> MFLNRLVKETSKAKRLFSMAQNNFARAGPYNPNRYKDYYIPRTLPKNEEIVEFVQSQHSVPASPIRNQRHINPVRESGPLPSYDGTYTMEDIRAVFYNTTVGRDYCYCQMDPEEIMRRVPGITRKEAEFITKLGLSPQEQVDFAYIAYNIGLDIFYF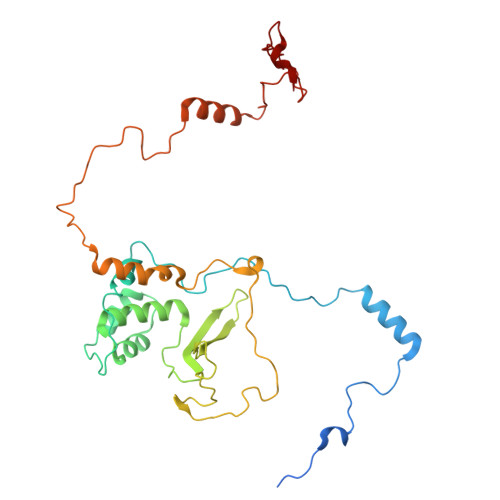TNQMFVARQVVTNSKGEKVEVLWNAQCYEDIAQLNVGFAPVLESVDYHWEIFLWADPPIKPNNDFDLNVPCTWFEYEQEWWMESCIQEDQFNLPEDERPYNTPRNPHCRKELWRSQDALQEEELMVNENWYPKNTQYNIYNQPDFIKPKSGSGAAADDIRI>GAMADIMAQADIALIGLAVMGQNLILNMNDHGFVVCAFNRTVSKVDDFLANEAKGTKVVGAQSLKEMVSKLKKPRRIILLVKAGQAVDDFIEKLVPLLDTGDIIIDGGNSEYRDTTRRCRDLKAKGILFVGSGVSGGEEGARYGPSLMPGGNKEAWPHIKTIFQGIAAKVGTGEPCCDWVGDEGAGHFVKMVHNGIEYGDMQLICEAYHLMKDVLGMAQDEMAQAFEDWNKTELDSFLIEITANILKFQDTDGKHLLPKIRDSAGQKGTGKWTAISALEYGVPVTLIGEAVFARCLSSLKDERIQASKKLKGPQKFQFDGDKKSFLEDIRKALYASKIISYAQGFMLLRQAATEFGWTLNYGGI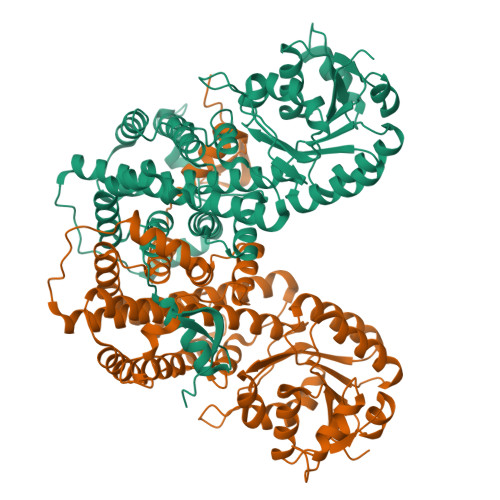ALMWRGGCIIRSVFLGKIKDAFDRNPELQNLLLDDFFKSAVENCQDSWRRAVSTGVQAGIPMPCFTTALSFYDGYRHEMLPASLIQAQRDYFGAHTYELLAKPGQFIHTNWTGHGGTVSSSSYNA[8x]>[4x]GSQQRKVLTLEKGDNQTFGFEIQTYGLHHREEQRVEMVTFVARVHESSPAQ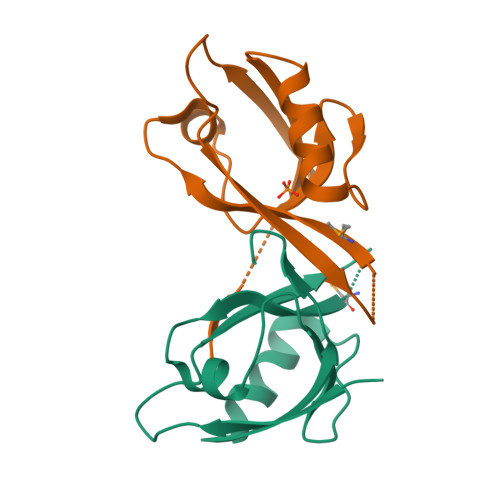LAGLTPGDTIASVNGLNVEGIRHREIVDIIKASGNVLRLETLYGTEESQL>[4x]MKAVQYTEIG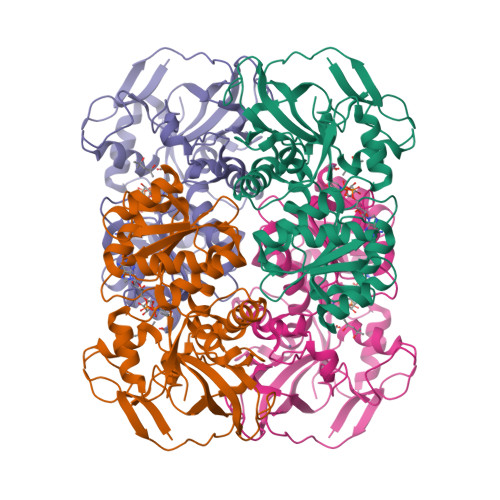SEPVVVDIPTPTPGPGEILLKVTAAGLCHSDIFVMDMPAAQYAYGLPLTLGHEGVGTVAELGEGVTGFGVGDAVAVYGPWGCGACHACARGRENYCTRAADLGITPPGLGSPGSMAEYMIVDSARHLVPIGDLDPVAAAPLTDAGLTPYHAISRVLPLLGPGSTAVVIGVGGLGHVGIQILRAVSAARVIAVDLDDDRLALAREVGADAAVKSGAGAADAIRELTGGQGATAVFDFVGAQSTIDTAQQVVAVDGHISVVGIHAGAHAKVGFFMIPFGASVVTPYWGTRSELMEVVALARAGRLDIHTETFTLDEGPAAYRRLREGSIRGRGVVVP>[2x]LPRETDEEPEEPGRRGSFVEMVDNLRGKSGQGYYVEMTVGSPPQTLNILVDTGSSNFAVGAAPHPFLHRYYQRQLSSTYRDLRKGVYVPYTQGKWEGELGTDLVSIPHGPNVTVRANI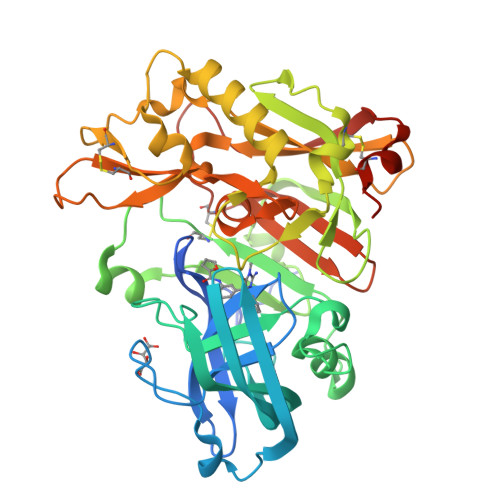AAITESDKFFINGSNWEGILGLAYAEIARPDDSLEPFFDSLVKQTHVPNLFSLQLCGAGFPLNQSEVLASVGGSMIIGGIDHSLYTGSLWYTPIRREWYYEVIIVRVEINGQDLKMDCKEYNYDKSIVDSGTTNLRLPKKVFEAAVKSIKAASSTEKFPDGFWLGEQLVCWQAGTTPWNIFPVISLYLMGEVTNQSFRITILPQQYLRPVEDVATSQDDCYKFAISQSSTGTVMGAVIMEGFYVVFDRARKRIGFAVSACHVHDEFRTAAVEGPFVTLDMEDCGYNIPQTDEST>[4x]QHWSYWLR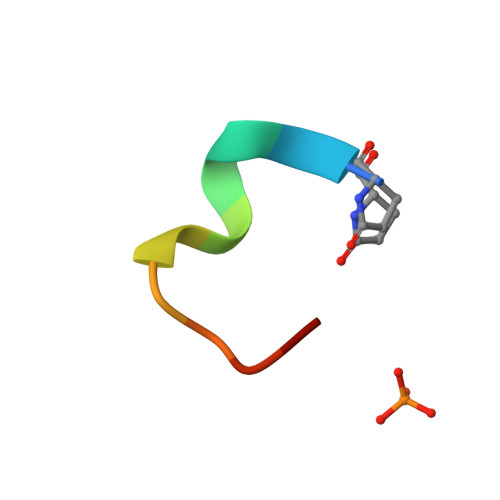PGX>[2x]FTFSPGQDIQLIPPLINLLMSIEPDVIYAGHDNTKPDTSSSLLTSLNQLGERQLLSVVKWSKSLPGFRNLHIDDQITLIQYSWMSLMVFGLGWRSYKHVSGQMLYFAPDLILNEQRMKESSFYSLCLTMWQIPQEFVKLQVSQEEFLCMKVLLLLNTIPLEGLRSQTQFEEMRSSYIRELIKAIGLRQKGVVSSSQRFYQLTKLLDNLHDLVKQLHLYCLNTFIQS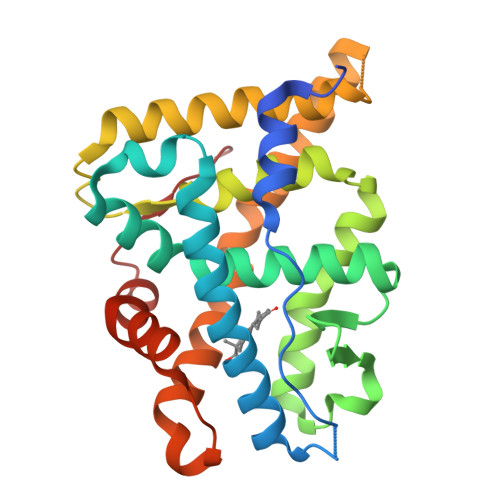RALSVEFPEMMSEVIAAQLPKILAGMVKPLLFHKK>[2x]FMDELVSLTYRSRVRLADPV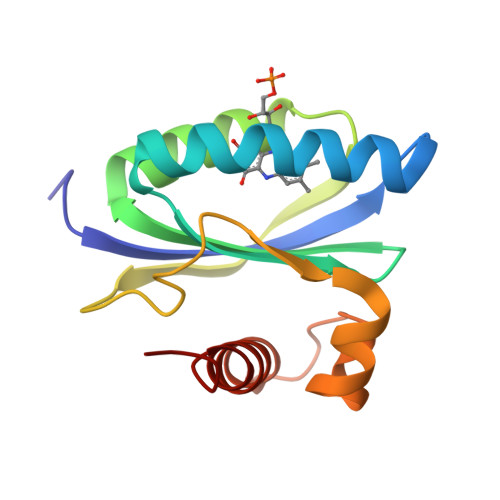ADIVQIMRASRVRNLRLGITGILLYNGVHFVQTIEGPRSACDELFRLISADPRHQEILAFDLEPITARRFPDWSMRIVSRKELRALAPDLERLDLSGPEDVAELHRTIAASLSRGDA> SNAMRGKMEFRVIIPARFDSTRLPGKALVDIAGKPMIQHVYESAIKSGAEEVVIATDDKRIRQVAEDFGAVVCMTSSDHQSGTERIAEAAVALGFEDDEIIVCLQGDEPLIPPDAIRKLAEDLDEHDNVKVASLCTPITEVDELFNPHSTKVVLNRRNYALYFSHAPIPWGRD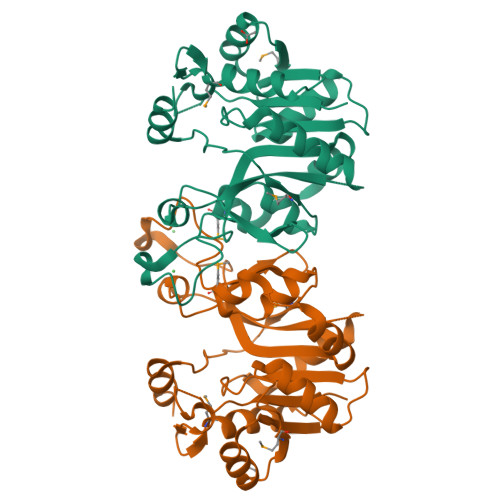TFSDKENLQLNGSHYRHVGIYAYRVGFLEEYLSWDACPAEKMEALEQLRILWHGGRIHMVVAKSKCPPGVDTEEDLERVRAYF>QSNAIWGLDRIDQRNLPLDRNYNANFDGFGVTAYVIDTG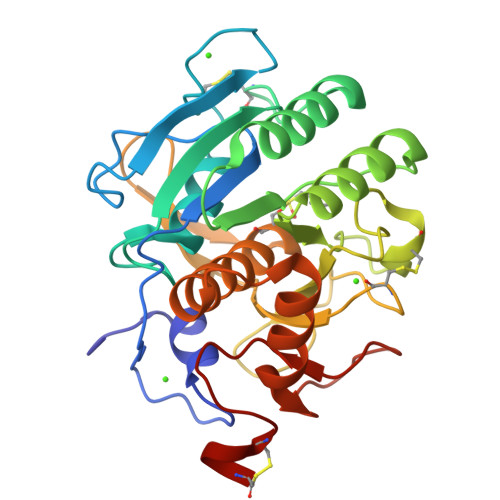VNNNHEEFGGRSVSGYDFVDNDADSSDCNGHGTHVAGTIGGSQYGVAKNVNIVGVRVLSCSGSGTTSGVISGVDWVAQNASGPSVANMSLGGGQSTALDSAVQGAIQSGVSFMLAAGNSNADACNTSPARVPSGVTVGSTTSSDSRSSFSNWGSCVDLFAPGSQIKSAWYDGGYKTISGTSMATPHVAGVAALYLQENNGLTPLQLTGLLNSRASENKVSDTRGTTNKLLYSLADSGCEPDCGGP[2x]>ADFAGAMKAFRGVVGAEWVFGDEEAVVPWSKTYIPDPAHQYKPVGAVCPQSVEEVQEIVRIANTYKQPLWTVSTGKNMGYGMTAPATPGQVVLDLKRMNRILEVDADLGTCLLEPGVTYQQLKDYLEEHKIPLWIDVPTVGPIASPVGNTLDRGVGYTPYGEHFMFQCGMEVCLPDGRLMRTGMGSIKGSTAWQAFKWGYGPYLDGLFTQSNFGIVTKMGLWLMPKPPVYKPFMVRHANMEDVPKIIEAMRPLRVSNLVANCNLMMSASYQLAMFKRRNEIVPDGAPLDEASLKKAASANGLGMWNTYFALYGTEQTVAGVEPIIRATLTASGGEVLTAAEMEGNPWFHHHQTLMQGGLNLDEVGLLRWRGAGGGLAWFAPVAAARGVEAERQTALAKEIVEKHGFDYTAAYAIGWRDLHHIIALLFDKADPTQEQKADACYRELVTRFGAQGWASYRTGVNSMDLVAQQYGEVNRDFNRTLKRAIDPNGILSPGKSGIHP[2x]

Enzymes of the vanillyl alcohol oxidase/p-cresol methyl hydroxylase (VAO/PCMH) superfamily are found across all kingdoms where they perform a range of metabolic functions. These flavoproteins share a conserved FAD-binding domain and a more variable substrate-binding domain that enables interactions with a range of substrates. One of these, the 4-phenol oxidases/dehydrogenases, catalyzes the oxidation of para-substituted phenolic compounds. A fundamental distinction is that the oxidases efficiently react with oxygen producing hydrogen peroxide whereas the dehydrogenases hardly react with oxygen and typically employ other proteins, such as cytochrome c, as acceptors.

The sequence and phylogenetic analysis additionally outlined a peculiar enzyme from Novosphingobium sp. that belongs to the EUGH clade and distinguishes itself for lacking a flavin-linking residue and the presence of a valine in the N5-interacting site. Thus, it represents an unusual family member that naturally binds the flavin non-covalently. The enzyme from Novosphingobium sp. was of particular interest because it was predicted to lack a covalent flavin and to feature an unusual Val/Thr pair around the flavin N5 site, beside sharing 43% and 36% sequence identity with VAD and VAO, respectively. The protein was expressed in high yields in E. coli and is thermally stable, with a melting temperature of 67 °C. Although it belongs to the EUGH clade, the enzyme is poorly active on eugenol whereas it converts vanillyl alcohol, with a kcat of 0.29 s-1. Moreover, its activity does not increase with the use of bovine heart cytochrome c as an artificial electron acceptor. The enzyme was therefore named as nsVAO, although we cannot exclude that it might use an endogenous cytochrome rather than oxygen as physiological substrate. Its crystal structure confirms that FAD is non-covalently bound, supporting the notion that removal of the covalent flavin linkage does not drastically affect the properties of VAO/PCMH enzymes. The protein exhibits a narrow tunnel leading of the flavin re side where Val181, homologous to Pro151 of VAD, is in direct contact with the N5 atom. The ability of nsVAO to use oxygen as electron acceptor thereby aligns with the oxidase activity observed for the P151V mutant of VAD.> MDKRIQEAVSLFEEVLIYGTERVIRSVDDPLWREYSPEQMQVLKLIYKEGEITSGRLAILQGVHKSAISNRLKKLIEKEVISIKPSGDKREKILVLTALGETVIKQSDAVLHEYIGKLMTNKVDDQEIEQFLVTFRKLKEILKM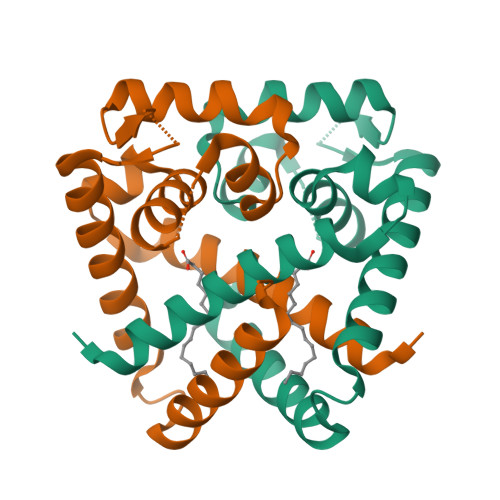NGV>KPVSLSYRCPCRFFESHVARAN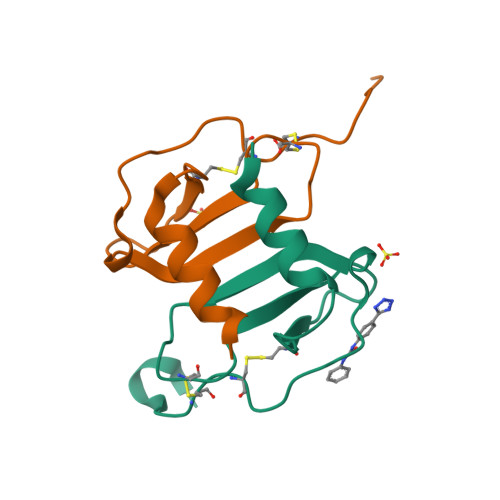VKHLKILNTPNCALQIVARLKNNNRQVCIDPKLKWIQEYLEKALNK[2x]> RRNVEARGIRRSPVVTPDIQIGHGEDAIEMDLYRYLLSNRIIFIGGYINDKMATQIVGSLMALEAVDENEDIRIYINSPGGQPYSVLGVVDAMQSIKPDVQTVALGACYSYASLVVAAGTKGKRYAMKNTRLMMTQPMGGSQGDIYQIKATVEELNALYQIFSRYYMKFTGMNQDQIEQATCRDHFMTPEQAKLEGLIDEIIRGKGDYTVPPAIVRQFREVGLVDDLTPGPFLKVDCN;>[3x]ARRSVAARSSAPELWTPTSEVKLAVSSRNPHPPVVCQGPPPPNPLVIERFQGVVSQLFQQRIVRLGGAVDDDMANLLVAQLLYLDSVDNKRDITMYVNSPGGSVTAGMAVFDTMRHIRPDVSTCCIGLAASMGAFILASGQAGKRYSLPNSRIMIHQPLGGAQGQATDIEIQANEILHHKLTLNGYLAQFTGQSMETITKDTDRDFFMSPQEAIEYGLVDAIISKPQMLQSREVALSS;>NSQPIVAPRTAEMQGDPFGLLLRQRIVFLGGEVEDFGADAIISQLLLLDSQDPTKDIKIFINSPGGSVTAGMGIYDAMMLCRADVNTYCFGLAASMGAFLLGAGKRGKRNSMPNSRIMIHQPLGGASGQAVDIEIQAKEIMYHKANLNRIMADYCQQPLSKIEEDTDRDRYMSPLEAKEYGLIDHIIGGEEAVFNVKGSLKKFPKIKEEFVTDKDDMVKRNIMDGDPFLSETPSWRFKSPQTEPYMPSQAPGSRWFRTRKVSKEDYKEMQEQRQAELMAESDDGKKSVKDRIDDAW[3x];>NYLDQGALNNESGRSLYRKQTERVIQEEESKKVFMIINSFGGSVGNGITVHDALQFIKAGSLTLALGVAASAASLALAGGTIGERYVTEGCHTMIHQPEGGLNGQASDIWIDSQEIMKIRLDVAEIYSLSTYRPRHKILRDLDRDFYLTAMETIYYGLADEIATNEVMHSIVEMTNQVWSYHDSKQERLLESRASLVGDSTQTQESNS[3x];> AYGDYPNYPEGRPLFLPEAERFGNPPDLPSLLLQQRVIYISMPFLPSVTELVVAQCY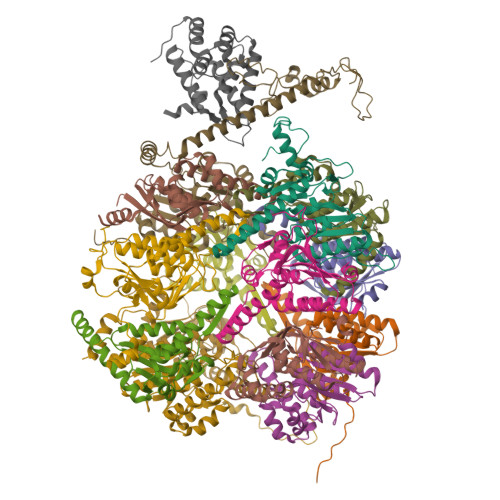YLDFDDRNRQRPIYVYLNSTGCINDKGQAISADNEFYAIWAALGFTRAPLYTGVTWKAQNQAAVLLSAGQKGHRYSFPHAKISTAPPVMNRVFGQAVDAQLQANELDYATKYYAAILARSTGKDLETCQKQYLSRKRYFSVKEAYEEGLVDKLVPGFMLNRFRKMQKDAGVGEEDLFDMNKPKFKFRRQ;> RKLSHLRKKLWKEAGPPPDLATRLFSERIMYLGMPIDSSVAELLTAQLFVLVQEAPDPIFFYINSTGIAKSTTKFGNEHEAIAVYSMMKGVQKYCPIYTLCVGNAFGEAALLLSAGSPGKRAALRSSTIMLRQPLQRLGGMQASDIDIYRKITREKTATMAKYLAACTKKTEEQIMTDFTRPRYFNPYEAVSYGLIDTVLEPKEERAVFKDWEKMGSEIADLGLWDDEEQPLPTNIMYPGTSQYWRSDFDG;> KKSPQGFWQVTTKQISAAKRSGAPKRKVTTMMPVSVPKVLCRPPGQRQSEWVDLWEAYTYQKVVFIKEAITEDVANNMIALTLYLDSLDQKRIYYWLNVPGGDVVPTLALYDTMQYVRSKTATVCYGLCLGMGGFLLTAGGEKGYRFAMPHSILMMHHPSGASRGQASEMHIESRELVRMRDYLSLLTSNATGQPYDRVIRELSRNKWMDPKQAIEYGMIDKVLTTPMPKMPSTGPSFKFERQNDELIGL;> LVVHARASRYDRRKPPPPDLPSLLFDQRIVYLGMPLVPAVTELMVAELLYLEKQGATLPIEMLINSSGTTRQDGEILSFDSEGVALTSTMGFIKNPISTVNMGLAVGWSCVVLSFGRKGWRKSLPHSLAMIQQPRVPPTGQRQAIEVHIKWREVLDYKRELLRMFSLGTGLPVDKLDADMQRPLYMRPQDALEYGIIDEIIEPNEDKAEKAAQYWIRSGRAESEGRLEQWQEYLSLQEEYALKDSFRKVMTQDLRAAYRDTSSKLLKNSSRNMEQVQEFKERLPDDMLTENDEVRLPFSRDGVKLAILNAECYAERNIARQVAANKVSVPDKWRAAYAARPAPAAPAAEVDYDALIRAVEAMDEKAFATTDLDTLVEQYRVPA;> ATATAAPSELDDVGVSAAAESIIQYAINFARASETYEVHSWMVLMGILKYETCTAAKILKSLGLEDLYGAWNEVLWALNVCDGLQPRSFVTDIKFADRAFKVITAASDFAVWHGKDKMYSEDVLMALAAGGVLEDLFPDLNLSFERVRKAVEKESGRRYQLPDETEEAGPLKSEDDVSFL> QYSSNTQQGRTSIVHLFEWRWV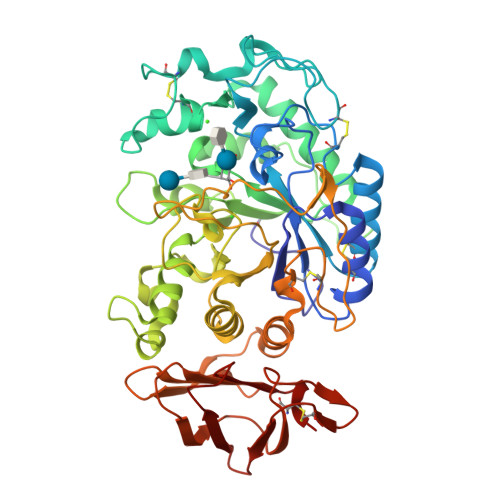DIALECERYLAPKGFGGVQVSPPNENVAIHNPFRPWWERYQPVSYKLCTRSGNEDEFRNMVTRCNNVGVRIYVDAVINHMCGNAVSAGTSSTCGSYFNPGSRDFPAVPYSGWDFNDGKCKTGSGDIENYNDATQVRDCRLSGLLDLALGKDYVRSKIAEYMNHLIDIGVAGFRIDASKHMWPGDIKAILDKLHNLNSNWFPEGSKPFIYQEVIDLGGEPIKSSDYFGNGRVTEFKYGAKLGTVIRKWNGEKMSYLKNWGEGWGFMPSDRALVFVDNHDNQRGHGAGGASILTFADARLYKMAVGFMLAHPYGFTRVMSSYRWPRYFENGKDVNDWVGPPNDNGVTKEVTINPDTTCGNDWVCEHRWRQIRNMVNFRNVVDGQPFTNWYDNGSNQVAFGRGNRGFIVFNNDDWTFSLTLQTGLPAGTYCDVISGDKINGNCTGIKIYVSDDGKAHFSISNSAEDPFIAIHAESKL> GGHAGTTYIFSKGGGQITYKWPPNDRPSTRADRLAIGFSTVQKEAVLVRVDSSSGLGDYLELHIHQGKIGVKFNVGTDDIAIEESNAIINDGKYHVVRFTRSGGN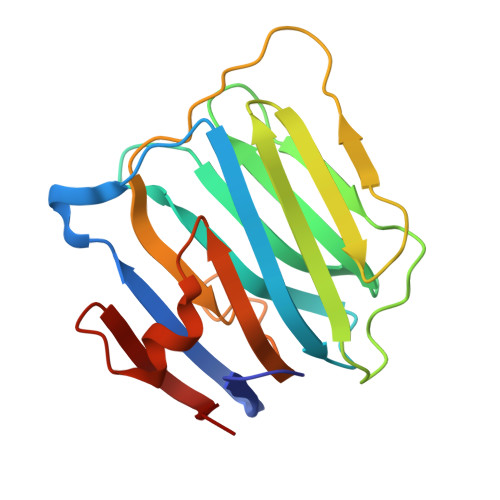ATLQVDSWPVIERYPAGRQLTIFNSQATIIIGGKEQGQPFQGQLSGLYYNGLKVLNMAAENDANIAIVGNVRLV> QFLFSMSTGPFICTVKDNQVFVANLPWTMLEGDDIQVGKEFAARVEDCTNVKHDMAPTCTKPPPFCGPQDMKMFNFVGCSVLGNK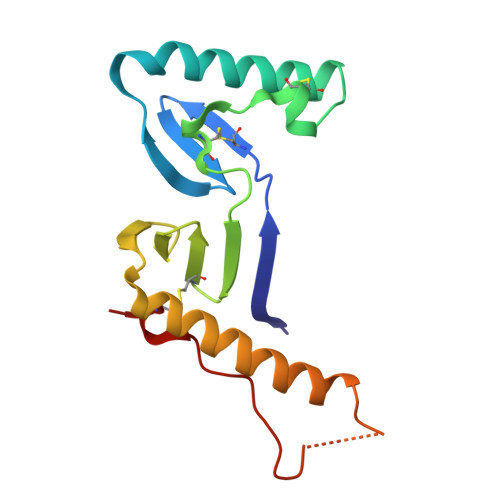LFIDQKYVRDLTAKDHAEVQTFREKIAAFEEQQENQPPSSGMPHGAVPAGGLSPPPPPSFCTVQ Compared to the RdRPs of other Flaviviridae representatives such as the NS5 of the Japanese encephalitis virus (JEV) and dengue virus (DENV) in the Flavivirus genus and the NS5B of the hepatitis C virus (HCV) of the Hepacivirus genus, the pestivirus NS5B contains a unique ∼90-residue N-terminal domain (NTD) that does not have notable sequence homology to any other viral or host proteins. The global conformation of our CSFV NS5B structures is consistent with the recently reported CSFV structure with an RMSD value of 0.9 Å (95% coverage) between the reported structure and our representative C-682 structure. These structures together reveal that the NTD adopts a globular α/β fold with an α-β-α-β-β-α pattern. The NTD interacts with the palm of the RdRP core intra-molecularly with a mixture of hydrophobic and hydrogen bonding interactions. Collectively, these biochemical data indicated that the RNA synthesis fidelity of CSFV NS5B is fine-tuned by its NTD through the intra-molecular interactions with the RdRP palm.

To better understand the nature of the NTD–RdRP intra-molecular interface interactions and whether they regulate the RdRP fidelity, we designed point mutations at the Y471 and E472 sites in the context of the WT NS5B and the N- and C-terminal deletion mutants. The other two structures, obtained using the C-672 construct bearing the Y471A-E472A double mutation (C-672_AA) and the C-672 construct with the E472A single mutation (C-672_E472A), were solved in a space group different from those of the WT, C-682 and C-672 structures. Very interestingly, the C-672_AA and C-672_E472A adopt a drastically different global conformation with the NTD–RdRP interface no longer maintained (C-672_AA structure shown in Figure 3D). The NTD–RdRP intra-molecular interactions are fully disrupted, and the NTD is rather involved in a non-intensive three-way interaction involving two symmetry-related neighboring NS5B molecules in the crystal lattice. As suggested by the two open conformation crystal structures (C-672_AA and C-672_E472A), the NTD–RdRP disengagement might occur in solution. In the chromatography analysis, the crystallographic open conformation C-672_AA and the C-672, or the AA mutant and the WT, had consistent retention volumes. By carefully comparing the proteolytic profiles at representative time points for all three constructs, the AA mutant also produced a few proteolytic products that either had obviously different amount from the WT or were consistent with the characteristic products of the N-91. These observations suggest that though the closed conformation is dominant for the AA mutant in solution, the open conformation AA mutant likely exists in solution as a minor fraction.

> MSNWVMQEENKQGNLTPLFEELLQQCPPGGQNKTAHMVSAYQLAQGNWMPTSCHVFMGTISARRTKTHPYEAYVKLRELVEEHKMKTLCPGSSLGKHNDWIIGKIKYQGNLRTKHMLNPGKVAEQLCREGHRHNVYNKTIGSVMTATGIRLEKLPVVRAQTDTTNFHQAIRDKIDKEENLQTPGLHKKLMEVFNALKRPELESSYDAVEWEELERGINRKGAAGFFERKNIGEILDSEKNKVEEIIDNLKKGRNIKYYETAIPKNEKRDVNDDWTAGDFVDEKKPRVIQYPEAKTRLAITKVMYKWVKQKPVVIPGYEGKTPLFQIFDKVKKEWDQFQNPVAVSFDTKAWDTQVTTKDLELIKDIQKYYFKKKWHKFIDTLTMHMTEVPVICADGEVYIRKGQRGSGQPDTSAGNSMLNVLTMVYAFCEATGVPYKSFDRVAKIHVCGDDGFLITERALGEKFASKGVQILAAAGKPQKITEGDKMKVAYQFDDIEFCSHTPIQVRWSDNTSSYMPGRNTTTILAKMATRLDSSGERGTIAYEKAVAFSFLLMYSWNPLIRRICLLVLSTELQVKPGKSTTYYYEGDPISAYKEVIGHNLFDLKRTSFEKLAKLNLSMSVLGAWTRHTSKRLLQDCVNMGVKEGNWLVNADRLVSSKTGNRYIPGEGHTLQGRGSSSHHHHHH> GSNQTNRTRRETSMRSAHPEFENKAVEIYTYSANSSEAEFSEDYLTVCPFERKIPGFSMSRVILNPEKYPLEREMVREKQVEMRQVLFCKENFSRVQKVLDFGCGHGTDVIQIAELYPHIKTHGFTITKAQAELGNQRIAQKNLGARAKIFNKDSSKDAFPDLYDMIVGIE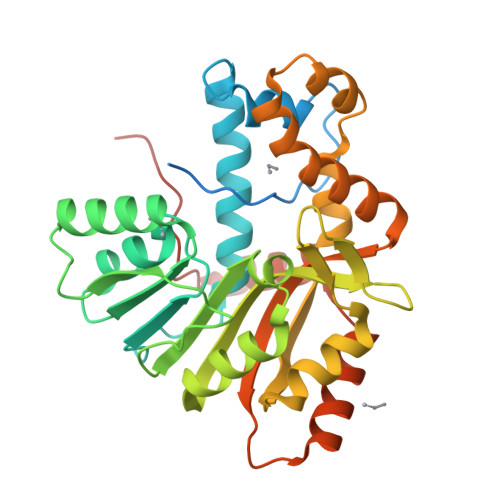VSFHIRNKHGLFQNISSSLNEEGTVLLIDYIANTRGPIVDQNVEVSIPTVQEWIELLAEHQLVIDEIIDVSPQIANALHDPDVEQYIKHLPKAVQDLYINTVNQSISLERGWISYCLFKLKKAPHLTYTKRCEWNASKLSKKRPYPEALAEMINSGYIPYPKQQTRTQPNPNA> IKELKMSKDEIKREYKEMEGSPEIKSKRRQFH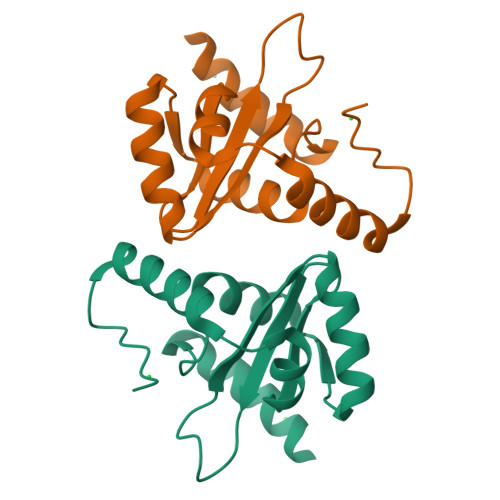QEIQSGNMRENVKRSSVVVADPTHIAIGILYKRGETPLPLVTFKYTDAQVQTVRKIAEEEGVPILQRIPLARALYWDALVDHYIPAEQIEATAEVLRWLERQNIEKQHSEML Deoxyribose-5-phosphate aldolases (DERAs) are acetaldehyde-dependent, Class I aldolases catalysing in nature a reversible aldol reaction between an acetaldehyde donor (C2 compound) and glyceraldehyde-3-phosphate acceptor (C3 compound, C3P) to generate deoxyribose-5-phosphate, DRP (C5 compound). The 3D structures of several DERA enzymes have been solved, and there are also a few complex structures available. These have revealed that despite of relatively low sequence identity, all DERA enzymes have the ubiquitous TIM (α/β)8-barrel fold where the catalytic amino acids as well as other amino acid residues around the active site seem to be relatively well conserved. The DERA reaction proceeds via Schiff base formation between an active site lysine residue (K167 in Ec DERA) and the donor acetaldehyde substrate. The active site of DERA is located in a deep binding cleft, where the donor acetaldehyde binds to the bottom of the cleft and the acceptor glyceraldehyde-3-phosphate to the upper part, near the cleft entrance.

The crystal structure of Ec DERA N21K variant, which had lowered specific activity on DRP, and wild-type like activity on DR and acetaldehyde, was determined with and without the ligand, D-2-deoxyribose-5-phosphate (DRP). The complex structure of Ec DERA N21K mutant revealed binding of the reaction product from DRP cleavage, i.e. glyceraldehyde-3-phosphate (C3P), to the acceptor site in one of the two protein molecules in the asymmetric unit. A similar conformational change in the loop around residue S238 in both the Ec DERA N21K mutant and wild-type structures can be seen upon glyceraldehyde-3-phosphate binding, when uncomplexed and complexed crystal structures are compared. In addition, in both N21K crystal structures, there are slight (about 0.2 to 0.4 Å) movements in the positions of altogether three active site loops containing residues G171, G204 and L20, respectively, when compared with the wild-type DERA crystal structure. The N21K mutation is located in the third loop. These small movements slightly narrow the access to the active site of the N21K variant and may thus contribute to the decreased activity against DRP in many of the N21K containing double mutants tested in this work. Most of these residues (i.e. G171, G204, S238 and S239, N21) are according to the structural data (by others and us, see also below) involved in binding the phosphate group of the glyceraldehyde-3-phosphate acceptor substrate.

>MTDLKASSLRALKLMDLTTLKDDDTDEKVIALCHQAKTPVGNTAAICIYPRFIPIARKTLKEQGTPEIRIATVTNFPHGNDDIDIALAETRAAIAYGADEVDVVFPYRALMAGNEQVGFDLVKACKEACAAANVLLKVIIETGELKDEALIRKASEISIKAGADFIKTSTGKVAVNATPESARIMMEVIRDMGVEKTVGFKPAGGVRTAEDAQKYLAIADELFGADWADARHYRFGASSLLASLLKALGH[2x]(2R)-3-hydroxy-2-(alpha-D-mannopyranosyloxy)propanoic acid | C9 H16 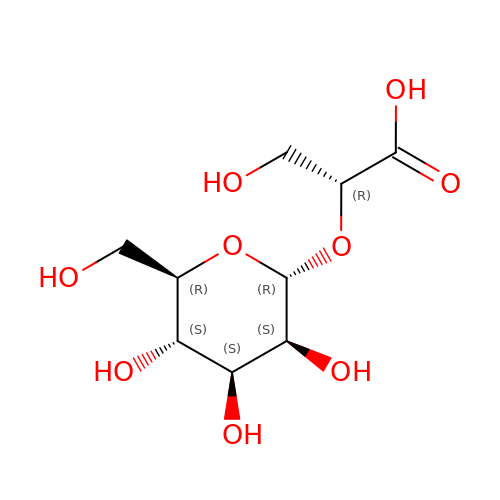O9 | DDXCFDOPXBPUJC-SAYMMRJXSA-N> MPSFNPVRFLELPIDIRKEVYFHLDGNFCGAHPYPIDILYKSNDVELPGKPSYKRSKRSKKLLRYMYPVFATYLNIFEYSPQLIEKWLEYAFWLRYDCLVLDCFKVNHLYDGTLIDALEWTYLDNELRLAYFNKASMLEVWYTFKEYKKWVIDSVAFDELDLLNVSNIQFNIDNLTPQLVDKCLSILEQKDLFATIGEVQFGQDEEVGEEKDVDVSGANSDENSSPSSTIKNKKRSASKRSHSDNGNVGATHNQLTSISVIRTIRSMESMKSLRKITVRGEKLYELL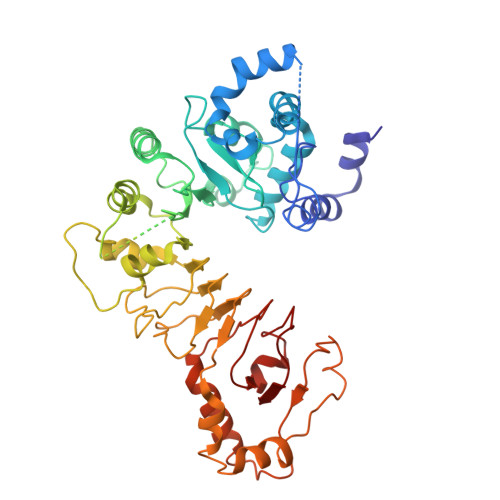INFHGFRDNPGKTISYIVKRRINEIRLSRMNQISRTGLADFTRWDNLQKLVLSRVAYIDLNSIVFPKNFKSLTMKRVSKIKWWNIEENILKELKVDKRTFKSLYIKEDDSKFTKFFNLRHTRIKELDKSEINQITYLRCQAIVWLSFRTLNHIKLQNVSEVFNNIIVPRALFDSKRVEIYRCEKISQVLVI> ASVKDTYTDRLDDWNGIIAGNQYYDSKNDQMAKLNQELEGKVADSLSSISSQADRIYLWEKFSNYKTSANLTATYRKLEEMAKQVTNPSSRYYQDETVVRTVRDSMEWMHKHVYNSEKSIVGNWWDYEIGTPRAINNTLSLMKEYFSDEEIKKYTDVIEKFVPDPEHFRKTTDNPFKALGGNLVDMGRVKVIAGLLRKDDQEISSTIRS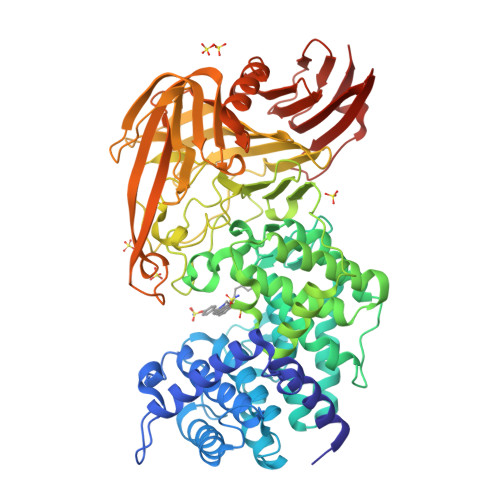IEQVFKLVDQGEGFYQDGSYIDHTNVAYTGAYGNVLIDGLSQLLPVIQKTKNPIDKDKMQTMYHWIDKSFAPLLVNGELMDMSRGRSISRANSEGHVAAVEVLRGIHRIADMSEGETKQRLQSLVKTIVQSDSYYDVFKNLKTYKDISLMQSLLSDAGVASVPRTSYLSAFNKMDKTAMYNAEKGFGFGLSLFSSRTLNYEHMNKENKRGWYTSDGMFYLYNGDLSHYSDGYWPTVNPYKMPGTTETDAKRADSDTGKVLPSAFVGTSKLDDANATATMDFTNWNQTLTAHKSWFMLKDKIAFLGSNIQNTSTDTAATTIDQRKLESSNPYKVYVNDKEASLTEQEKDYPETQSVFLESSDSKKNIGYFFFKKSSISMSKALQKGAWKDINEGQSDKEVENEFLTISQAHKQNGDSYGYMLIPNVDRATFNQMIKELESSLIENNETLQSVYDAKQGVWGIVKYDDSVSTISNQFQVLKRGVYTIRKEGDEYKIAYYNPETQESAPDQEVFKKLEQHHHHHH>[5x]MATNIESTLHISDLILQASP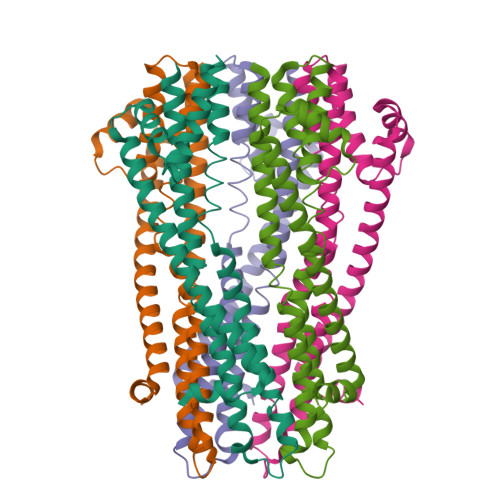VVQLVMLILLLASIFSWYLIAKLHMSYKKARQDDEHFQKMFWSGAELNTLYNNAQLNSKRSGLEDIFYQGLSEFFKLKKRQAPTSQMIEGTERILRVGLSRDQGSLEYGLGTLASIGSVAPYIGLFGTVWGIMNAFIGLAAVDQVTLATVAPGIAEALIATAIGLFAAIPAVLAFNHFTAKSESVYSDRALFAEEMIALLQRQSVGSSQEDA> GPHMLEHSGISQASEYDDPPGLREKAEYLLREWVNLYHSAAAGRDSTKAFSAFVGQMHQQGILKTDDLITRFFRLCTEMCVEISYRAQAEQQHNPAANPTMIRAKCYHNLDAFVRLIALLVKHSGEATNTVTKINLLNKVLGIVVGVLLQDHDVRQSEFQQLPYHRIFIMLLLELNAPEHVLETINFQTLTAFCNTFHILRPTKAPGFVYAWLELISHRIFIARMLAHTPQQKGWPMYAQLLIDLFKYLAPFLRNVELTKPMQILYKGTLRVLLVLLHDFPEFLCDYHYGFCDVIPPNCIQLRNLILSAFPRNMRLPDPFTPNLKVDMLSEINIAPRILTNFTGVMPPQFKKDLDSYLKTRSPVTFLSDLRSNLQVSNEPGNRYNLQLINALVLYVGTQAIAHIHNKGSTPSMSTITHSAHMDIFQNLAVDLDTEG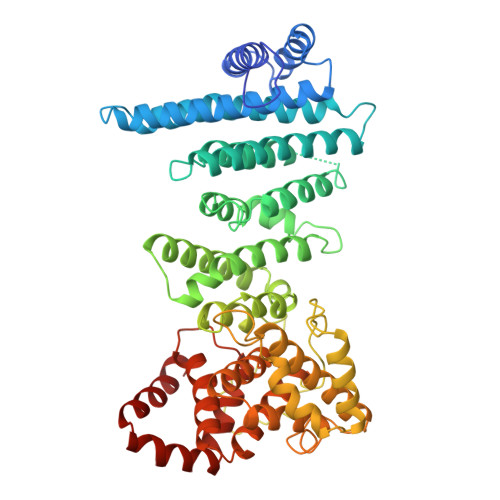RYLFLNAIANQLRYPNSHTHYFSCTMLYLFAEANTEAIQEQITRVLLERLIVNRPHPWGLLITFIELIKNPAFKFWNHEFVEEEPEIEKLFQSVAQCCM>[4x]GSVESHPVLEKLKAAHSYNPKEFEWNLKSGRVFIIKSYSEDDIHRSIKYSIWCSTEHGNKRLDSAFRCMSSKGPVYLLFS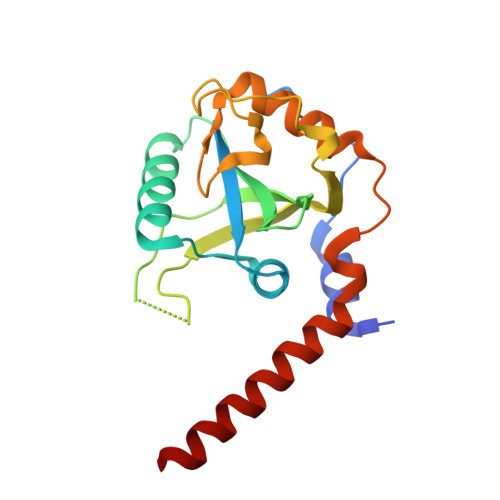VNGSGHFCGVAEMKSPVDYNTSAGVWSQDKWKGKFDVQWIFVKDVPNNQLRHIRLENNDNKPVTNSRDTQEVPLEKAKQVLKIISSYKHTTSIFDDFAHYEKRQEEEEVVRKERQSRNKQ> MGWDLTVKMLAGNEFQVSLSSSMSVSELKAQITQKIGVHAFQQRLAVHPSGVALQDRVPLASQGLGPGSTVLLVVDKSDEPLSILVRNNKGRS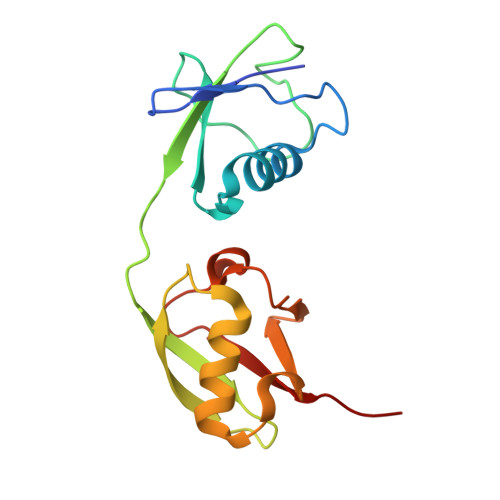STYEVRLTQTVAHLKQQVSGLEGVQDDLFWLTFEGKPLEDQLPLGEYGLKPLSTVFMNLRLRG>[4x]MAFSIPPL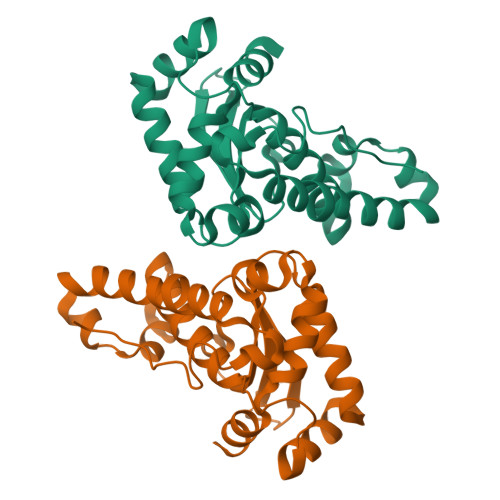PWGYDGLAAKGISKEQVTFHYDKHHMGYVTKLNAAANSNPALAAKSVEEIIRTEKGPIFNLAAQIFNHNFYWESMSPNGGGEPSGKLAEAIRASFGSFAKFKEEFTNAAVGHFGSGWAWLVQDTTTKKLKVFQTHDAGCPLTEADLKPILTCDVWEHAYYIDYKNDRPAYVQTFWNVVNWDHAENQFTR>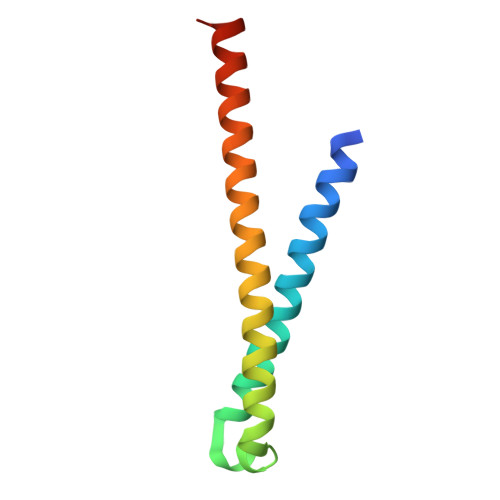 GSHMAPADYFRVLVQQFEVQLQQYRQQIEELENHLATQANNSHITPQDLSMAMQKIYQTFVALAAQLQSIHENVKVLKEQYLSYRKMFLGDAG> HDDHDHDHAHGSLGKHEHGVAQLNVALDGKTLELELDSPAMNLVGFEHAASTDADKAAVAKARAQLEKPLELFALPVTAGCSVASQELRSPLFGDKAPAHAHKEKAGHEHEHEHEHEHGHADIHAHYQLSCEKPELLKLLTLAEFFKRFPATQKIQVQLIGPDGQKGADLAPASAELKL

The structural and zinc-binding properties of PA4063, one of the periplasmic proteins expressed by Pseudomonas aeruginosa under zinc-deficient conditions, are presented. PA4063 has a noncanonical ferredoxin-like fold. Two zinc-binding sites with micromolar affinity are exposed and are located on the same face of the structure. Two histidine-rich loops, which are disordered in the apoprotein, contribute to zinc coordination in one of the sites. These findings strongly suggest a role for PA4063 in zinc trafficking, possibly acting as a metal chaperone or as a regulator of a transport system.

The structure of PA4063 in complex with zinc was solved by soaking crystals in zinc acetate solution since crystallization did not occur in presence of zinc. Later, a higher resolution (2.85 Å) data set was collected from a zinc-soaked tetragonal crystal, confirming the positions of the two zinc-binding sites and allowing a better determination of the complex geometry and coordination distances. Site a is located on the flat surface of the β-sheet in correspondence with the histidine residues. The same mode of binding is detected in all three monomers of the hexagonal crystal: besides His124 and His126, the zinc ion binds to Glu87, likely as a monodentate ligand, and a water molecule, adopting a tetrahedral coordination geometry. The water molecule is not visible in the tetragonal crystal, where zinc appears to be coordinated by only three ligands. Comparison with the apo structure shows that coordination requires rearrangement of the donor side chains, which move closer to the site, while Glu35 is displaced. Site b is about 20 Å from site a, on the edge of the β-sheet where the His-rich sequences are inserted. Notably, a few residues belonging to these sequences, which are disordered in apo PA4063, become structured and take part in zinc coordination, although some variability is present. As for site a, the coordination is tetrahedral and three donor groups are provided by one glutamate, Glu47, and two histidines, His16 and His18. The fourth donor was modelled as a water molecule in monomer A of the hexagonal crystal, while in monomers B and C, as well as in the tetragonal crystal, the electron-density map indicates His120 to be the donor.>[4x]GSHMIRIDATPYPYQFHP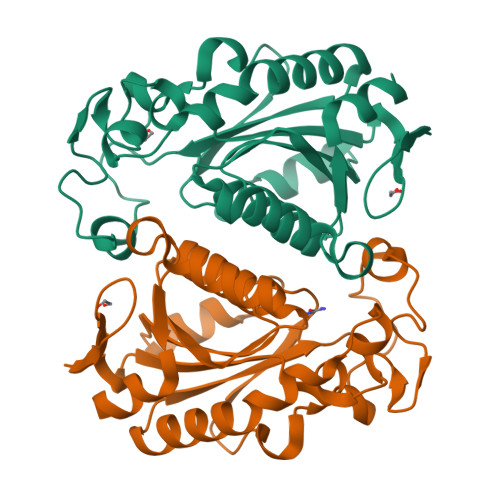RSTALVVIDMQRDFIEEGGFGSALGNDVRPLAAIVPTVAALLQLAREAGMLVVHTRESHLPDLSDCPRSKRLRGNPTLGIGDVGPMGRILVQGEPGNQILPQLAPVEGELVIDKPGKGAFYATDLHAQLQERRITHLLVAGVTTEVSVQTSMREANDRGYECLVIEDACASYFPDFHRITLEMLTAQGGIVGWRTPLAQLQAGVA> SNAMEKKPIAFKVPPNSK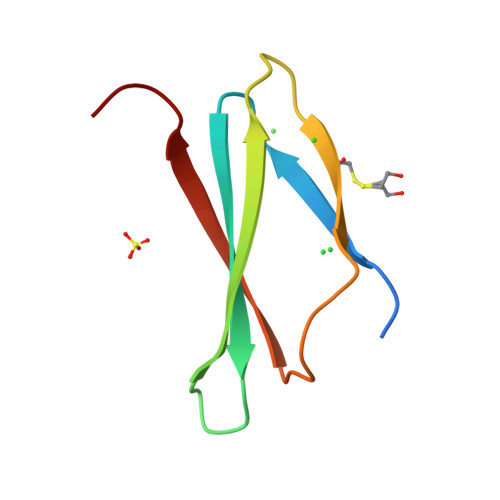LKVTFFGPYNEVITNVSIINQLSTPKCQTITRYPNYTKYETEVRSLSSC> GSHGQYLLPEAKAQDSDKICVVINLDETLVHSSFKPVNNADFIIPVEIDGVVHQ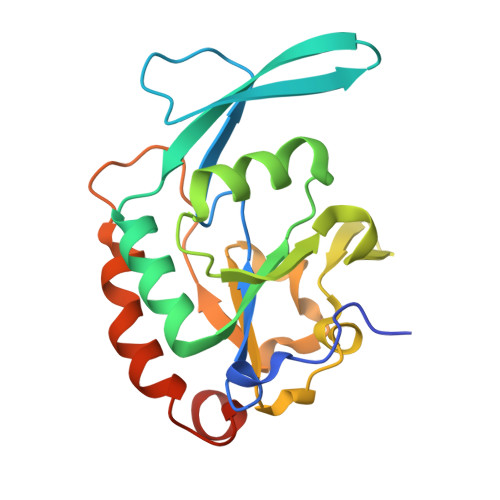VYVLKRPHVDEFLQRMGELFECVLFTASLAKYADPVADLLDKWGAFRARLFRESCVFHRGNYVKDLSRLGRDLRRVLILDNSPASYVFHPDNAVPVASWFDNMSDTELHDLLPFFEQLSRVDDVYSVLRQPRPGS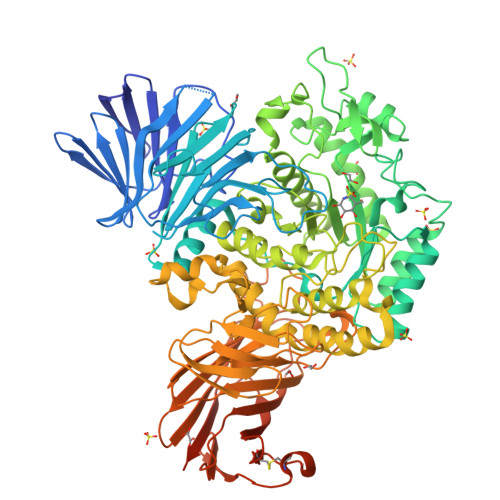> MNPVKREIHPDAVFYKEHKLRNDGLVITTNQGNIRLQFKSEAAIEVLYRADSKQLPSFALAQPESAIKAQLTETENHLQFSGGTLTARIQKRPFAISYYRDSELLLAEESGFQVNTDKINFRFYLSPGEKILGGGQRILGMDRRGQRFPLYNRAHYGYSDHSGQMYFGLPAIMSSKQYILVFDNSASGAMDIGKTESDILQLEAKSGRSAYILVAGNSYPSLIENFTQVTGRQPLPPRWALGSFASRFGYRSEAETRATVQKYKTEDFPLDTIVLDLYWFGKDIKGHMGNLDWDKENFPTPLDMMADFKQQGVKTVLITEPFVLTSSKRWDDAVKAKALAKDPQGQPKAFELYFGNGGIIDVFSKEGSRWFSSIYKDLSKQGVAGWWGDLGEPEMHPEDTQHAIGDADTVHNAYGHRWAEMLYQQQLDQFPELRPFIMMRAGFVGSQRYGMIPWTGDVSRTWGGLASQVELALQMSLLGFGYIHSDLGGFADGETLDKEMYIRWLQYGVFQPVYRPHGQDHIPSEPVFQDEETKAILRPLVKLRYRMLPYIYTAAYQNTLTGMPLMRPLFFSDEKNPALIDNKTSYFWGDSLLVTPITQAGVESVSIPAPKGVWFDFWKDTRYQTDGAPLTLPTDLHTIPVLVKAGAFMPYVPAVSTTEDYRSDSLEIHYYADASVPLAQGEIFEDDGKDPNSIKRNQFDLLTLQATHTDNQLHFQLARTGKGYRGMPERRATTLVIHNASDQYQHLDINGKTIAIAQADCASTPALACYDQERRQLQLVFTWGREALNLRLHKGGRADPAFLYKVVINSKLEGKPIPNPLLGLDSTRTGHHHHHH>MTDTPFIRPDMKAFLEAIAAMAGPTLAEMTLEEARASYVALHGMADRPARELAVIRNLSCPGPAGDIPLRLYDARESREAGPVITFYHGGGFVIGDLDTHHNLCTEIAALMDLPVVAVDYRLAPEHPFPAAIEDCEAATRWVASSPSELGRTASGVIPIGDSAGGNATIVVSQLLGAKPADVPVVLQVPIFPLASDAVGSASLEAFAEGFVLTKASIEFFDTAYKADRADPRGFPILGDHTAAPPTIVATASLDPIRDSGRDYAKALVEAGRDVVYLEMEGVTHSFTNIRAAVPSTQGDLERIIAAMKMMLGTA[3x];> MTDTPFIRPDMKAFLEAIAAMAGPTLAEMTLEEARASYVALHGMADRPARELAVIRNLSCPGPAGDIPLRLYDARESREAGPVITFYHGGGFVIGDLDTHHNLCTEIAALMDLPVVAVDYRLAPEHPFPAAIEDCEAATRWVASSPSELGRTASGVIPIGDSAGGNATIVVSQLLGAKPADVPVVLQVPIFPLASD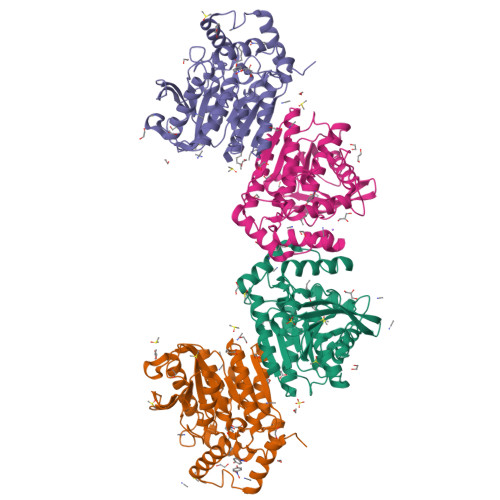AVGSASLAAFAEGFVLTKASIEFFDTAYKADRADPRGFPILGDHTAAPPTIVATASLDPIRDSGRDYAKALVEAGRDVVYLEMEGVTHSFTNIRAAVPSTQGDLERIIAAMKMMLGTA>GMTPIAQRDGQAIQLVGFDGDDTLWKSEDYYRTAEADFEAILSGYLDLGDSRMQQHLLAVERRNLKIFGYGAKGMTLSMIETAIELTEARIEARDIQRIVEIGRATLQHPVEVIAGVREAVAAIAADYAVVLITKGDLFHQEQKIEQSGLSDLFPRIEVVSEKDPQTYARVLSEFDLPAERFVMIGNSLRSDVEPVLAIGGWGIYTPYAVTWAHEQDHGVAADEPR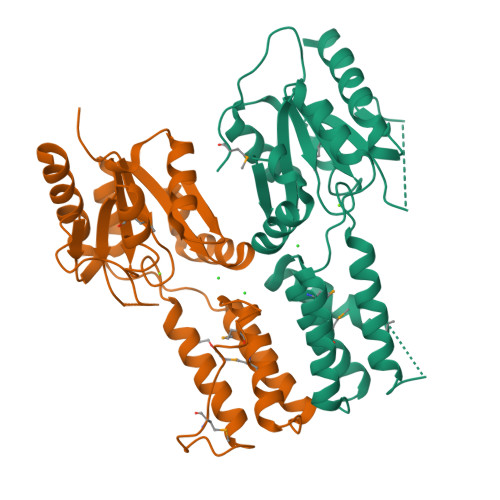LREVPDPSGWPAAVRALDAQAGRQQ[2x]>[4x]GPLGSSKTKPFTLPILTISEMSNSRFPVPIDSLHTSPTENIVVQCQNGRVTLDGELMGTTQLLPSQICAFRGTLTRSTSRASDQADTPTPRLFNYYWHIQLDNLNGTPYDPAED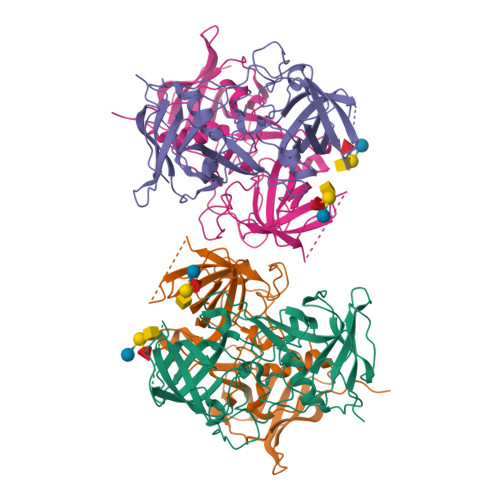IPAPLGTPDFRGKVFGVASQRNPDSTTRAHEAKVDTTSGRFTPKLGSLEITTESDDFDPNQPTKFTPVGVGVDNEAEFQQWSLPNYSGQFTHNMNLAPAVAPNFPGEQLLFFRSQLPSSGGRSNGVLDCLVPQEWVQHFYQESAPAQTQVALVRYVNPDTGRVLFEAKLHKLGFMTIAKNGDSPITVPPNGYFRFESWVNPFYTLAPMGTGNG> GSMA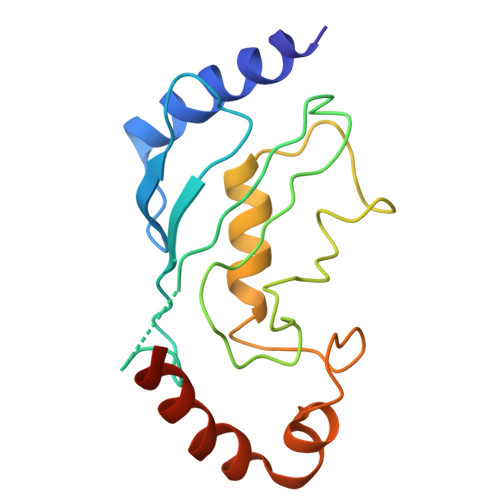ASRRLMKELEEIRKCGMKNFRNIQVDEANLLTWQGLIVPDNPPYDKGAFRIEINFPAEYPFKPPKITFKTKIYHPNIDEKGQVCLPVISAENWKPATKTDQVIQSLIALVNDPQPEHPLRADLAEEYSKDRKKFCKNAEEFTKKYGEKRPVD>[2x]GPHMQTLTLSPNLIGFNSNEGEKLLLTSRSREDFFPLSMQFVTQVNQAYCGVASIIMVLNSLGINAPETAQYS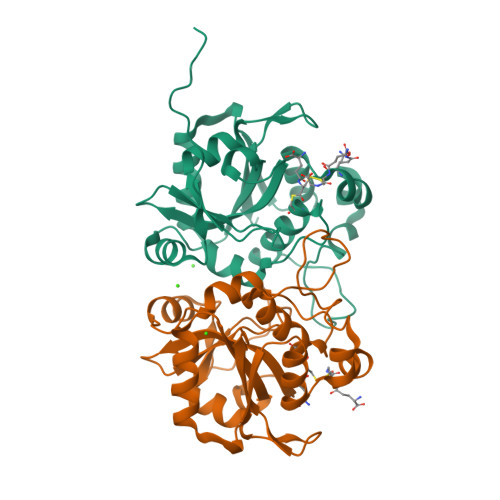PYRVFTQDNFFSNEKTKAVIAPEVVARQGMTLDELGRLIASYGVKVKVNHASDTNIEDFRKQVAENLKQDGNFVIVNYLRKEIGQERGGHISPLAAYNEQTDRFLIMDVSRYKYPPVWVKTTDLWKAMNTVDSVSQKTRGFVFVSKTQD1-{2-deoxy-3,5-O-[(4-iodophenyl)(phosphono)methylidene]-beta-D-threo-pentofuranosyl}-5-methylpyrimidine-2,4(1H,3H)-dione | C17 H18 I N2 O8 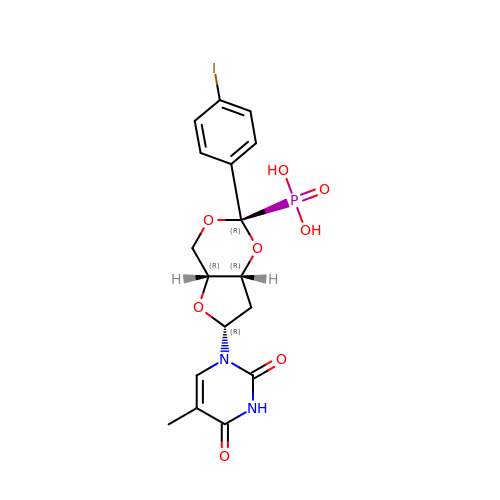P | CXQVVVNMWAGPGY-VMUDFCTBSA-N>[2x]MRFQVIVAAATITMITSYIPGVASQSTSDGDDLFVPVSNFDPKSIFPEIKHPFEPMYANTENGKIVPTNSWISNLFYPSADNLAPTTPDPYTLRLLDGYGGNPGLTIRQPSAKVLGSYPPTNDVPYTDAGYMINSVVVDLRLTSSEWSDVVPDRQVTDWDHLSANLRLSTPQDSNSYIDFPIVRGMAYITANYNNLTPQFLSQHAIISVEADEKKSDDNTSTFSGRKFKITMNDDPTSTFIIYSLGDKPLELRKQDNSNLVASKPYTGVIRVAKLPAPEFETLLDASRAVWPTGGDISARSDDNNGASYTIKWKTNSNEAPLLTYAYAHHLTSIDDSNVKRTDMTLQSATKGPMTALVGNEWTLRETELSPVEWLPLQAAPNPTTINEIMTEINKDIASNYTQ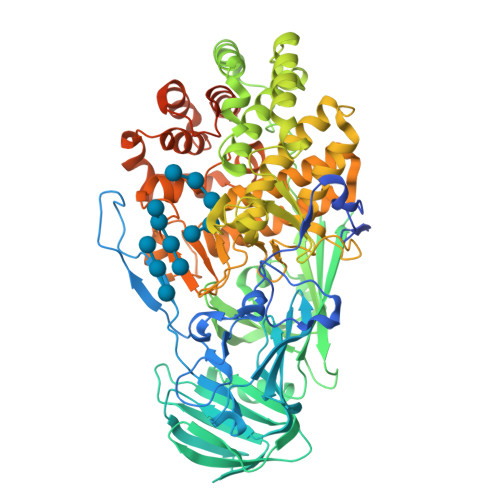ETAKEDNYFSGKGLQKFAMLALILNKSDQTQLRNPELAQIALDKLKAAFLPYLQNEQADPFRYDTLYKGIVAKAGLPTSMGGTDDLSAEFGHSYYSDHHYHQGYFVVTAAIIHHLDPTWNADRLKAWTEALIRDVNNANDGDEYFAAFRNWDWFAGHSWAGGIKPDGALDGRDQESVPESVNFYWGAKLWGLATGNTPLTKLASLQLAVTKRTTYEYFWMLDGNKNRPENIVRNKVIGIYFEQKTDYTTYFGRFLEYIHGIQQLPMTPELMEYIRTPEFVSQEWDEKLGAIAPTVQSPWAGVLYLNYAIINPAEAYPALRKVQMDDGQTRSYSLYLTATRPHFFRRSLLAALARHGSTRRPSLPSSGDDDKHEDGFLLRFRRLNPFNLKHRIY> NNIDFDSIAKMLLIKYKDFILSKFKKAAPVENIRFQNLVHTNQF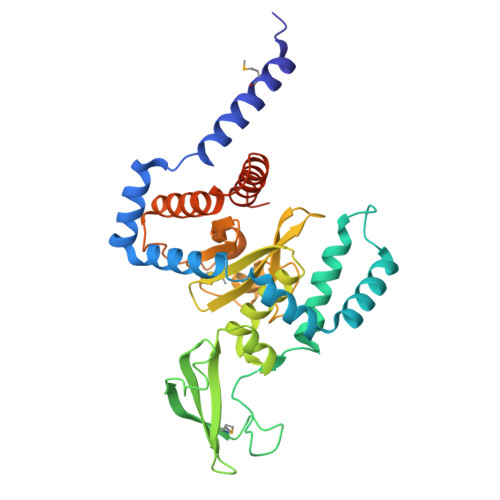AQGVLGQSQHLCTVYDNPSWHSIVLETLDLDLIYKNVDKEFAKDGHAEGENIYTDYLVKELLRYFKQDFFKWCNKPDCNHCGQNTSENMTPLGSQGPNGEESKFNCGTVEIYKCNRCGNITRFPRYNDPIKLLETRKGRCGEWCNLFTLILKSFGLDVRYVWNREDHVWCEYFSNFLNRWVHVDSCEQSFDQPYIYSINWNKKMSYCIAFGKDGVVDVSKRYILQNELPRDQIKEEDLKFLCQFITKRLRYSLNDDEIYQLACRDEQEQIELIRGKTQETKSESVSAASKS> MGSSHHHHHHSSGENLYFQGHMSELKQDQYWMQQAIELAKRGLYSTKPNPNVGCVIVKDDQLIGEGFHPKAGQPHAEVFALRQAGEQAQGATAYVTLEPCAHYGRTPPCAEALVKAQVKKVVVACPDPNPLVAGKGVQILKNAGIEVEIGICEDLAAKLNQGFLKAMSTGMPYVRLKVASSLDGRTAMASGESKWITGSAARQDVQHWRAISGAVITGIDTVIADDCQLNVRSLHNIDIETVAQPKRVILDRRGRLPLTAKILENPETVMVMGPYRQELADLGVIQLEIQPLKTLLQTLSKQYQIYDVLIEAGATLSSAFLQEGLIDEMISYVAPTLLGQSARAMFNADFEYMAQQLRFKLLDVIQLDQDIRLRLIPTQEKV

We selected a bifunctional enzyme, diaminohydroxyphosphoribosylaminopyrimi­dine deaminase (EC 3.5.4.26)/5-amino-6-(5-phosphoribosylamino)­uracil reductase (EC 1.1.1.193), called RibD, in this pathway as a potential target in Gram-negative bacteria. In bacteria, the second and third stages of this metabolic process involve zinc-dependent deamination and an NADPH-dependent reduction at the ribosyl group, respectively. RibD is constructed from an N-terminal deaminase domain, which carries a Zn2+ ion, and a C-terminal NADPH-binding reductase domain. The overall structure of AbRibD is an arch-like dimer and most certainly not a uniform globular entity.

The second form, which crystallized in space group P43212, has one subunit in the asymmetric unit, with a crystallographic twofold generating the same dimer as observed in form I. Both crystal forms have an estimated Matthews coefficient of 3.2 Å3 Da−1 and a solvent content of about 60%. The exception is oxalate, which was observed in crystal form II. Oxalate is a common contaminant of polyethylene glycols owing to polymer breakdown and crystal form II was obtained in the presence of polyethylene glycol 8000. In form II, the side chain of Arg84 is oriented away from the active site, while His81 adopts a conformation intermediate between the two observed in form I. All residues interacting with the oxyanions are strictly conserved in RibD sequences, with the exception of Arg84, which is sometimes replaced by lysine. In crystal form II Trp174 is not visible in the electron density, suggesting a degree of flexibility in this part of the active site consistent with the altered positions noted in form I. Crystal form II was obtained in the presence of 5 mM GMP, which had been added as a potential substrate analogue for the deaminase reaction. Unexpectedly, a GMP molecule was observed in the NADPH-binding site of the reductase domain, occupying the adenine-binding pocket. There are no direct hydrogen bonds involving the purine moiety and the enzyme; rather, it is positioned by van der Waals interactions with Leu271 and Leu295 on one side and the side chain of Arg231 on the other. A second GMP, refined with an occupancy of 0.5, was observed positioned in a depression on the surface of the protein formed between α7 and β14 (data not shown) and distant from either active site. We do not think that the GMP binding we observe is of biological relevance; rather, it is a consequence of the crystallization conditions with the high level of GMP present.> AQLTDEEKYRDCERFKCPCPTCGTENIYDNVFDGSGTDMEPSLYRCSNIDCKASPLTFTVQLSNKLIMDIRRFIKKYYDGWLICEEPTCRNRTRHLPLQFSRTGPLCPACMKATLQPEYSDKSLYTQLCFYRYIFDAECALEKLTT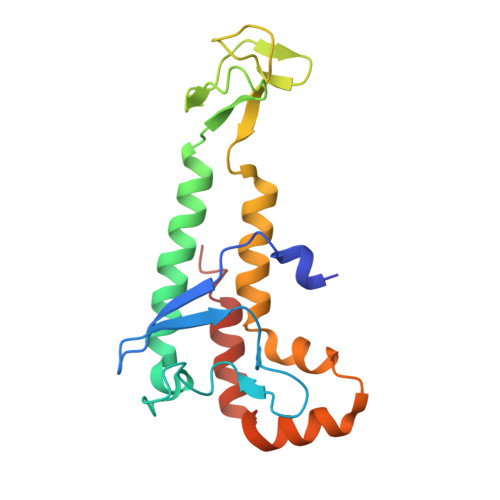DHEKDKLKKQFFTPKVLQDYRKLKNTAEQFLSRS> GSFTPRTAHILKPLMSPPSREEIVAT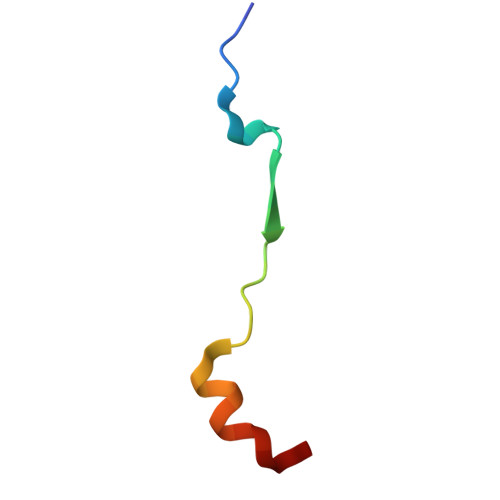LLDH> MKHHHHHHHHGGLVPRGSHGASAPALTKSQTDRLEVLLNPKDEISLNSGKPFRELESELLSRRKKDLQQIYAEERENYLGKLEREITRFFVDRGFLEIKSPILIPLEYIERMGIDNDTELSKQIFRVDKNFCLRPMLTPNLYNYLRKLDRALPDPIKIFEIGPCYRKESDGKEHLEEFTML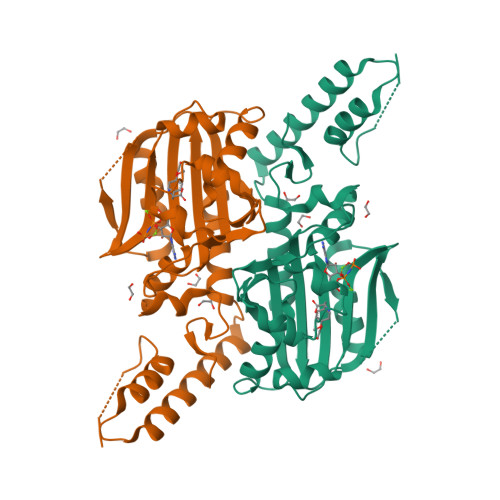VFWQMGSGCTRENLESIITDFLNHLGIDFKIVGDSCMVFGDTLDVMHGDLELSSALVGPIPLDREWGIDKPWIGAGFGLERLLKVKHDFKNIKRAARSESYYNGISTNL>GGGVGVSTGSYDNQTHYKFLGDGWVEITAYSTRMVHLNMPKSENYCRVRVHNTNDTGTASHMAMDDAHEQIWTPWSLVDANAWGVWFQPSDWQYISNNMIHINLHSLDQELFNVVIKTVTEQNTGAEAIKVYNNDLTAAMMVALDSNNILPYTPAIDNQETLGFYPWKPTIPSPYRYYFSCDRNLSVTYKDEAGTITDTMGLASGLNSQFFTIENTQRINLLRTGDEYATGTYYFDTEPIRLTHTWQTNRHLGQPPQITELPSSDTANATLTARGYRSGLTQIQGRNDVTEATRVRPAQVGFCQPHDNFETSRAGPFKVPVVPADITQGLDHDANGSLRYTYDKQHGQSWASQNNKDRYTWDAVNYDSGRWTNNCFIQSVPFTSEPNANQILTNRDNLAGKTDIHFTNAFNSYGPLTAFPHPAPIYPQGQIWDKELDLEHKPRLHTQAPFVCKNNAPGQLLVRLAPNLTDQYDPNSS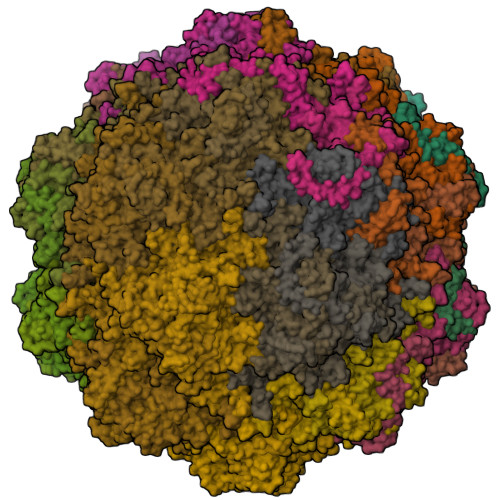NLSRIVTYGTFFWKGKLTLKAKMRPNATWNPVFQISATNQGTNDYMSIERWLPTATGNITNVPLLSRPVARNTY[60x]1-(beta-D-glucopyranosyl)-5-(hept-1-yn-1-yl)pyrimidine-2,4(1H,3H)-dione | C17 H24 N2 O7 | 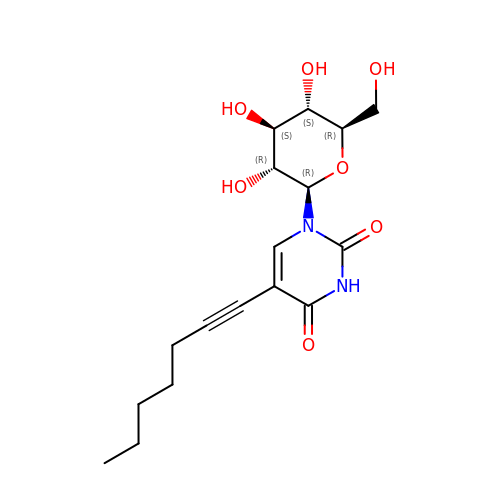ZIAKFTYLGUACKB-XYFZXANASA-N>MTHHYPTDDIKIKEVKELLPPIAHLYELPISKEAS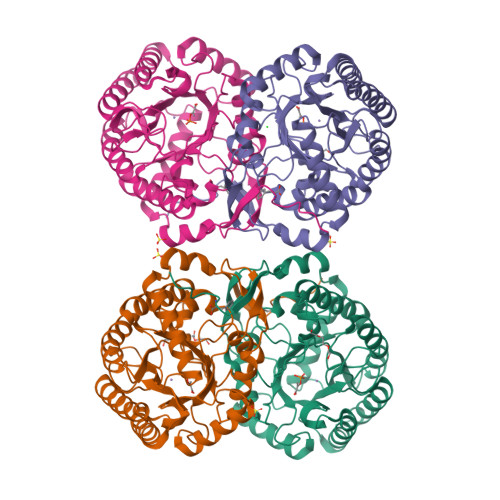GLVHRTRQEISDLVHGRDKRLLVIIGPCSIHDPKAALEYAERLLKLRKQYENELLIVMRVYFEKPRTTVGWAGLINDPHLDGTFDINFGLRQARSLLLSLNNMGMPASTEFLDMITPQYYADLISWGAIGARTTESQVHRELASGLSCPVGFKNGTDGNLKIAIDAIGAASHSHHFLSVTKAGHSAIVHTGGNPDCHVILRGGKEPNYDAEHVSEAAEQLRAAGVTDKLMIDCSHANSRKDYTRQMEVAQDIAAQLEQDGGNIMGVMVESHLVEGRQDKPEVYGKSITDACIGWGATEELLALLAGANKKRMARAS[4x]>[2x]SEFENPLKQLLAEEQWEFEVTAFYRGRQVFQQTLFCPGGLRLVGSTADMTLPWQPVTLPDPEGFLTDKLVKEYVGQVLKGLGNGLALWQAGQCLWAQRLGHSHAFWALGEELLPDSGRGPDGEVHKDKDGAVFDL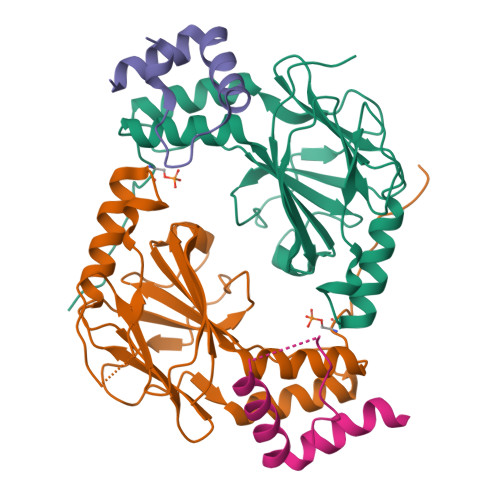RPFVADLIAFMEGSGHSPRYTLWFCMGEMWPQDQPWVKRLVMVKVVPTCLKELLEMAREGGASSLKTVDLHISNS;>SALQDLLRTLKSPSSPQQQQQVLNILKSNPQLMAAFIKQRTAKYVAN[2x]> GHMRSMVSKGEELIKENMRMKVVMEGSVNGHQFKCTGEGEGNPYMGTQTMRIKVIEGGPLPFA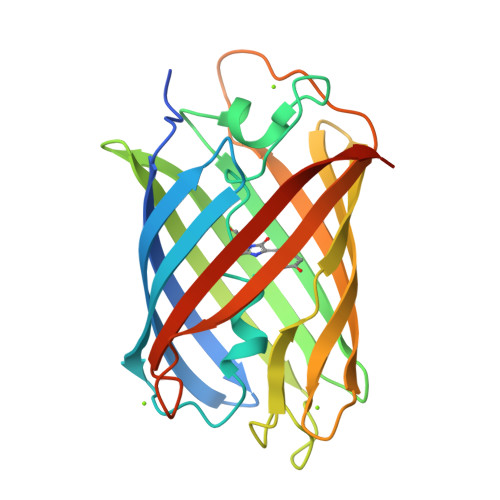FDILATSFLYGSRTFIKYPKGIPDFFKQSFPEGFTWERVTRYEDGGVVTVMQDTSLEDGCLVYHVQVRGVDFPSNGPVMQKKTKGWEPSTEMMYPADGGLRGYTHMALKVDGGGHLSCSFVTTYRSKKTVGNIKMPGIHAVDHRLERLEESDNEMFVVLREHSVAKFAGRGGMDELYK>GIDPFTATIARKGEGSVLEQIDQGSILKLPSNLLFENATSDAINQDMMLYIERIAKIIQKLPKRVHINVRGFTDDTPLVKTRFKSHYELAANRAYRVMKVLIQYGVNPNQLSFSSYGSTNPIAPNDSLENRMKNNRVEIFFSTDANDLSKIH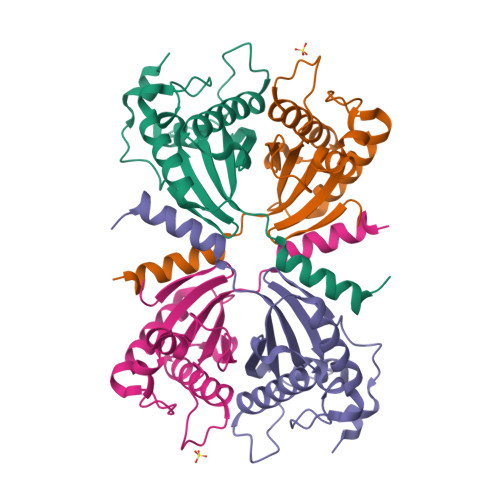SILDNEFNPHKQQE[2x]> GAMGKGQCRVWIITTNMGVESVPTCRHSKLGEPSKTIQEVIEALKPLFEKRPVWTRRALLNHLDPSYTHYLKFALPYLSYLWTSGPFRDTYTRFGYDPRKDSNAAAYQALFFKLKLNGKHKGTKTHVFDGKTLFPTNRVYQVC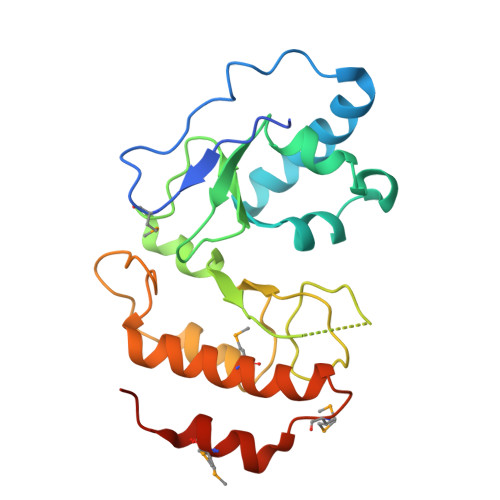DIVDPTIAPLLKDTQLRSECHRDTGWYRSGRYYKVRDLMREKLFALIEGEMPSEVAVNMILNAEEVEESDRY> IAT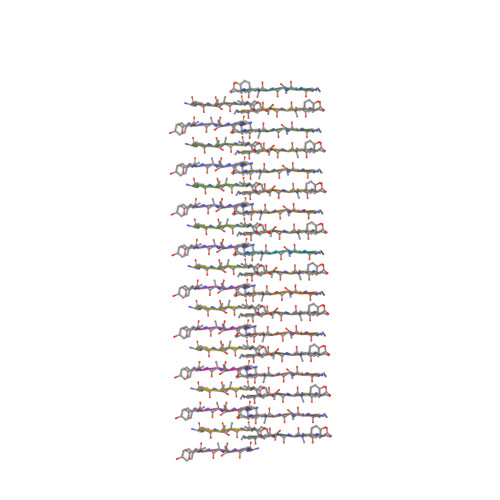LYV>MGHHHHHHSHDSHDLQRFLSDFRDLMSWINGIRGLVSSDELAKDVTGAEALLERHQEHRTEIDARAGTFQAFEQFGQQLLAHGHYASPEIKQKLDILDQERADLEKAWVQRRMMLDQCLELQLFHRDCEQAENWMAAREAFLNTEDKGDSLDSVEALIKKHEDFDKAINVQEEKIAALQ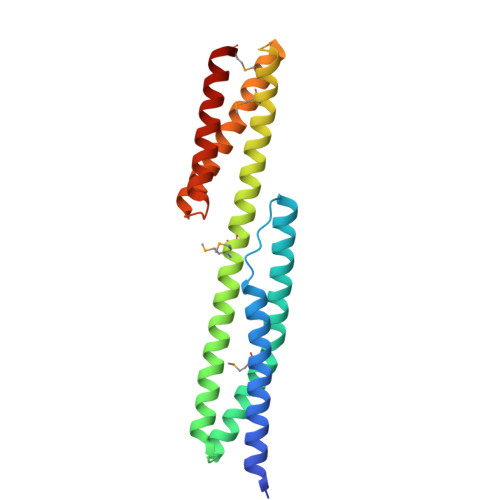AFADQLIAAGHYAKGDISSRRNEVLDRWRRLKAQMIEKR[2x]(3Z)-N-ETHYL-N-METHYL-2-OXO-3-(PHENYL{[4-(PIPERIDIN-1-YLMETHYL)PHENYL]AMINO}METHYLIDENE)-2,3-DIHYDRO-1H-INDOLE-6-CARBOXAMIDE | C31 H34 N4 O2 | 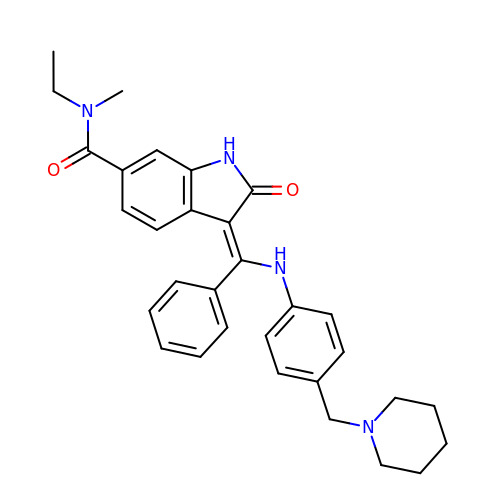MUSRTIADFPCYTQ-ZIADKAODSA-N Polyomaviruses are small double-stranded DNA (dsDNA) viruses with a circular genome of approximately 5,000 bp. All glycan-binding polyomaviruses analyzed to date engage oligosaccharide (glycan) structures featuring terminal sialic acids that in mammals are usually presented either on gangliosides, which are molecules composed of a glycosphingolipid, i.e., a ceramide and an oligosaccharide, or on glycoproteins, which contain mostly complex and branched oligosaccharides attached to amino acids during co- and posttranslational modification steps. These sialylated glycan structures interact with loop regions at the outer margin of the major capsid protein VP1, at the apical surface of the polyomavirus capsid, as revealed by X-ray crystallography and cryoelectron microscopy. The VP1 surface exhibits an astonishing plasticity, providing virus-specific interactions for a range of Neu5Ac linkage types and further specific characteristics of Neu5Ac-containing glycans.

In order to enable an understanding of their structural features and receptor-binding strategies, we expressed and purified VP1 pentamers of NJPyV and HPyV12 and solved X-ray structures of both native and liganded proteins. The two pentamers lack N- and C-terminal residues, which renders them assembly incompetent but does not affect the structure of the VP1 surface loops and binding of sialylated ligands. As expected, both proteins feature the conserved jelly-roll fold typical for polyomavirus VP1. Our structure-based sequence analysis shows that the BC2 loop of HPyV12, which essentially mediates all interactions with Neu5Ac, is especially highly conserved in several animal viruses. In HPyV12 VP1, the BC2 loop comprising the Neu5Ac-binding site is formed by amino acids T69 to Q83 (T73 to E87 in TSPyV VP1), whereas the putative binding sites in ShPyV VP1, GhPyV VP1, and FiPyV VP1 include amino acid residues T61 to Q75, T57 to E71, and T58 to E72, respectively. Cα atoms of the BC2 loop (residues 67 to 82) from the liganded HPyV12 VP1 structure superpose with the respective residues of the native structure with an RMSD of 0.3 Å (55), indicating that the Neu5Ac docks into a preformed binding pocket within the BC2 loop and that no conformational changes occur upon ligand binding.

>[5x]GSHMGGIEVLDVKTGDDSITQIEAFLNPRMGVNDETNTWYGFSEQVTVATARETDRPPKEQMPYYSCARIPLPLLNEDMTCNTLLMWEAVSVKTEVIGSNTLMNVHDYMTRTDNGVGHPVVGSTYHMFAVGGEPLDLQGIQQSHLVQYPEGLIVPKSVTDVTAKIQCLDPSAKAKLDKDGKYPIETWSPDPSRNENTRYFGNYYGGLTTPPVLTFTNTVTTILLDENGVGPLCKGDGLFLSCCDVMGWFTAGSGTHQRFRGLPRYFNVQLRKRAVRN>[2x]GIDPVEQSKVDLSMNDQIWQLLDTLSRHENAWPFRKP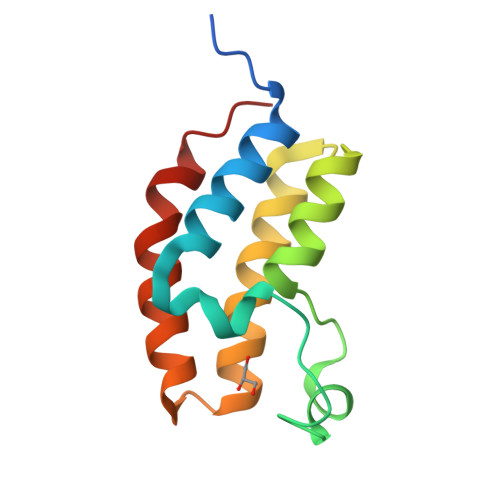VSIGEASDYYEIIKEPTDIQTMKRKAKNKEYKTLSEFSSELKRMFDNCRFYNAKNTIYTKYANQLEAFIWPMLQTIQES>GPPGPPGPPGVPGEAGPPGPPGPP[6x];>[4x]GAMDARSVNGEFPRHVKLKNEIENLLDQVTQLYTKHNSNYQQYNAQAGRLDLRQKAEYLKGLNDWAERLLQELNGEDVKKVLGKVAFEKDDLEKEVKELKEKIDKKEKEYQDC

The M protein is an essential virulence factor of *Streptococcus pyogenes*, or group A streptococcus (GAS), one of the most common and dangerous human pathogens. Encoded by the chromosomal *emm* gene, the M protein is covalently anchored at its C-terminus to the cell wall, covering the GAS surface at high density and acting as an adhesin and a potent immune evasion factor. The M3 protein is produced by the prevalent *emm*3 GAS serotype, which is frequently associated with severe invasive diseases. To gain insights into mechanism and biological role of streptococcal collagen binding, we characterised the interaction of M3 with the Collagen Ligand Collections (CLCs, triple-helical collagen peptide libraries formerly known as Toolkits), and determined crystal structures of the M3 N-terminal domain (M3-NTD), encompassing the HVR, alone and in complex with a CLC-derived collagen peptide.

To increase chances of crystallization, a shorter 24-residue peptide, JDM238, was synthesized which contains the GVOGEA motif flanked by three glycine-proline-4-hydroxyproline (GPO) repeats at each terminus. Crystals formed in conditions containing JDM238 and M3-NTD at a 3:2 molar ratio and diffracted synchrotron X-rays to 2.3 Å resolution. In agreement with our ITC data for CLC II-27 binding to M3-NTD, the M3-NTD dimer is bound to two copies of triple-helical JDM238. While both copies occupy equivalent binding sites on opposite faces of the M3-NTD T-bar, they contact the protein with two different regions ([Fig fig7]). One copy contacts M3-NTD through residues 15-21 of the C-terminal GPO repeats, the other is bound at its more central GPOGVO region (residues 6-12) ([Fig fig7] and [Fig fig8]). The presence of two different binding registers in the same crystal is likely an effect of crystal packing, as this binding mode results in a compact assembly required for crystallization ([Fig fig7]—figure supplement 1), but it also reflects a lack of specificity of collagen binding by M3, in line with the CLC screening data. The M3 collagen binding site includes the PARF region on H2 (residues 94-101), extending beyond it to include the C-terminal half of H1 and most of H2 ([Fig fig8]). Interfaces between the binding partners largely comprise hydrophobic interactions between highly complementary surfaces. M3 residues Tyr96 and Trp103 play prominent roles: they pack against Hyp and Pro sidechains, filling grooves on the collagen triple helices and form polar contacts with the peptide backbone. The indole amino group of Trp103 interacts with the carbonyl of Ala15 or Hyp6 (depending on the register), while Tyr96 forms a water-mediated hydrogen bond with the carbonyl of Hyp9 or Hyp18.3-[4-chloranyl-3-(2-methylphenoxy)naphthalen-1-yl]-6-(trifluoromethyl)-5~{H}-pyrimidine-2,4-dione | C22 H14 Cl F3 N2 O3 | 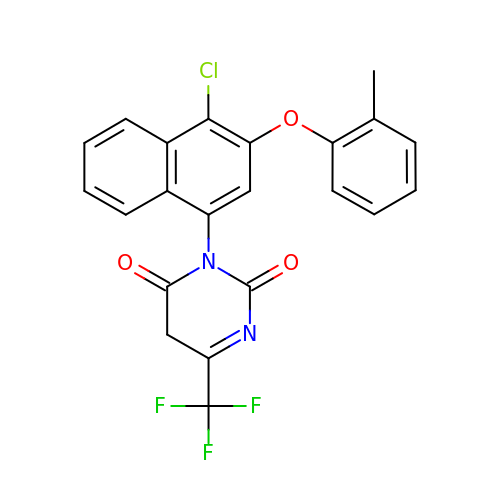PRDYNMSOAPXRSB-UHFFFAOYSA-N>[2x]MKETTIFAMHLGKALDPNLPVFVKAEKDTNIKLVNVASQNQTDQIQAYNLMLTEGKLPDIVSYELSADLENLGIEGGLIPLEDLINQHAPNLKKFFEENPRY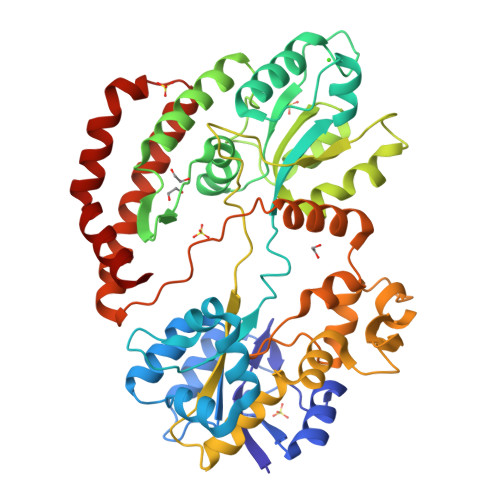KKDAVAVDGHIYMIPNYYDYFNIKVSQGYFIRQDWLEKLGLKEPRTVDELYTTLKAFREKDPNGNGKKDEVPFFVRANNVRKVLTSLVDLFKASPIWYEENGMVKYGPAQKEFKHAIKELSKWYKEGLIDEEIFTRGLESRDYLLSNNLGGATDDWIASTSSYNRNLADKIPGFNLKLVLPYELNGNAKTRHARTTYLGGWGISKDAKDPVSLIKYFDYWYSVEGRRLWNFGIEGSEYTLVDGKPVFTDKVLKNPDGKTPLAVLREVGAQYRLGAFQDAQYELGWASESAKAGYKYYMDNDVVLDELPILKYTKEKSKEFVSIDTAMRAVVEEKAQQWILGSGDIDKEWDAYIKRLENLGLSKAEQIQNEAF>MAFAISKRNATLFLVTLLLISVPLSSSTLQQDFVKCLVDNSDVSFPITASFFSPDQNATLFKEELESTAQNLRYLTPSNPKPVFIFEPLYETHVQAAVVCAKKLQLHLRLRSGGHDYEGLSFVAEDETPFVIVDLSKLRQVDVDLDSNSAWAHAGATIGEVYYRIQEKSQTHGFPAGLCSSLGIGGHLVGGAYGSMMRKFGLGADNVLDARIVDANG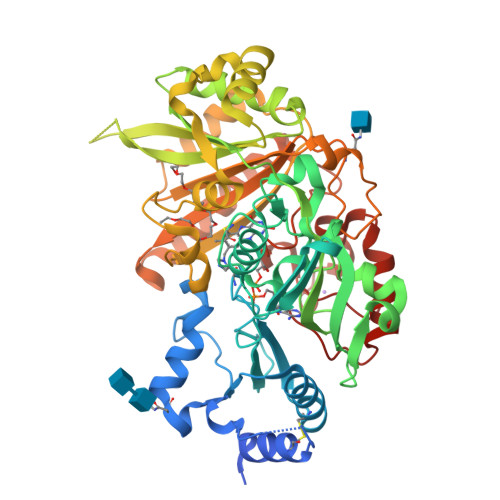QILDRAAMGEDVFWAIRGGGGGSFGVILAWKIKLVPVPATVTVFTVTKTLEQDGTKVLYKWEQIADKLDDDLFIRVIISPASKTTKPGNRTISMSYQAQFLGDSNRLLQVMQKSFPELGLTKKDCTEMSWIKSVMYIAGFPNSAAPEALLAGKSLFKNHFKAKSDFVKEPIPVEGLEGLWERFLEEDSPLTIWNPYGGMMSRISESEIPFPHRNGTLFKIQWLSTWQDGKVSEERHMKWIREMYSYMEQYVSKNPRQAYVNYRDLDLGTNEGETDAREWGAKYYKGNFERLVKIKGEFDPDNFFRHEQSVPTKIG[2x]>AMRQCAIYGKGGIGKSTTTQNLVAALAEMGKKVMIVGCDPKADSTRLILHSKAQNTIM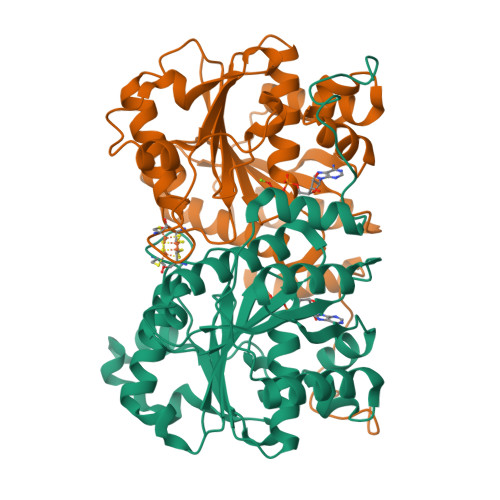EMAAEAGTVEDLELEDVLKAGYGGVKCVESGGPEPGVGCAGRGVITAINFLEEEGAYEDDLDFVFYDVLGDVVCGGFAMPIRENKAQEIYIVCSGEMMAMYAANNISKGIVKYANSGSVRLGGLICNSRNTDREDELIIALANKLGTQMIHFVPRDNVVQRAEIRRMTVIEYDPKAKQADEYRALARKVVDNKLLVIPNPITMDELEELLMEFGIMEVEDESIVGKTAEEV[4x]> ESSRSAMMYIQELRSGLRDMHLLSCLESLRVSLNNNPVSWVQTFGAEGLASLLDILKRLHDEKE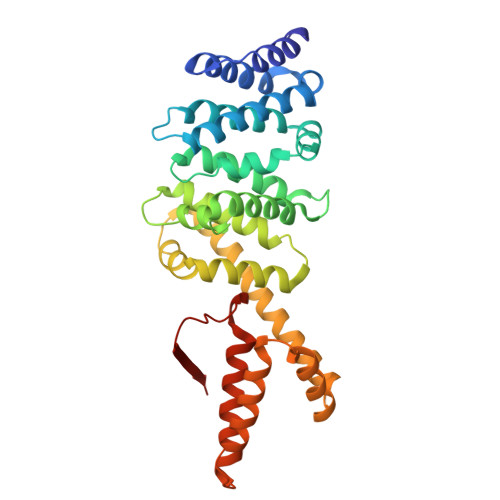ETSGNYDSRNQHEIIRCLKAFMNNKFGIKTMLETEEGILLLVRAMDPAVPNMMIDAAKLLSALCILPQPEDMNERVLEAMTERAEMDEVERFQPLLDGLKSGTSIALKVGCLQLINALITPAEELDFRVHIRSELMRLGLHQVLQELREIENEDMKVQLCVFDEQGDEDFFDLKGRLDDIRMEMDDFGEVFQIILNTVKDSKAEPHFLSILQHLLLVRNDYEARPQYYKLIEECVSQIVLHKNGTDPDFKCRHLQIDIERLVD> MSNISRQAYADMFGPTVGDKVRLADTELW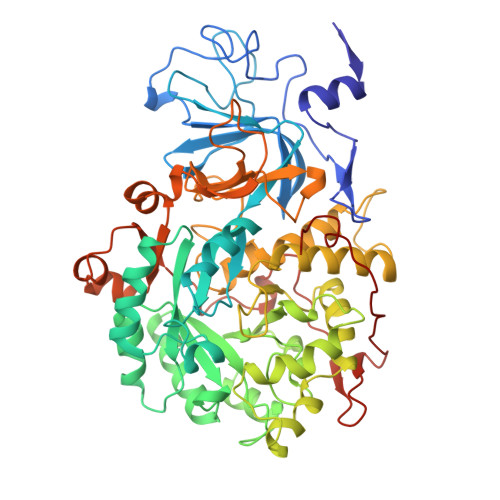IEVEDDLTTYGEEVKFGGGKVIRDGMGQGQMLAADCVDLVLTNALIVDHWGIVKADIGVKDGRIFAIGKAGNPDIQPNVTIPIGAATEVIAAEGKIVTAGGIDTHIHWICPQQAEEALVSGVTTMVGGGTGPAAGTHATTCTPGPWYISRMLQAADSLPVNIGLLGKGNVSQPDALREQVAAGVIGLKIHEDWGATPAAIDCALTVADEMDIQVALHSDTLNESGFVEDTLAAIGGRTIHTFHTEGAGGGHAPDIITACAHPNILPSSTNPTLPYTLNTIDEHLDMLMVCAHLDPDIAEDVAFAESRIRRETIAAEDVLHDLGAFSLTSSDSQAMGRVGEVILRTWQVAHRMKVQRGALAEETGDNDNFRVKRYIAKYTINPALTHGIAHEVGSIEVGKLADLVVWSPAFFGVKPATVIKGGMIAIAPMGDINASIPTPQPVHYRPMFGALGSARHHCRLTFLSQAAAANGVAERLNLRSAIAVVKGCRTVQKADMVHNSLQPNITVDAQTYEVRVDGELITSEPADVLPMAQRYFLF>MSPISRHHHHHHLVPRGSASLRANDAPIVLLHGFTGWGREEMFGFKYWGGVRGDIEQWLNENGYRTYTLAVGPLSSNWDRACEAYAQLVGGTVDYGAAHAAKHGHARFGRTYPGLLPELKRGGRIHIIAHSQGGQNARMLVSLLENGSQEEREYAKAHNVSLSPLFEGGHHFVLSVTTIATPHDGTTLVNMVDFTDRFFDLQKAVLEAAAVASNVPYTSQVYDFKLDQWGLRRQPGESFDHYFDRLKRSPVWTSTDTARYDLSVSGALKLNQWVQASPNTYYLSFSTERTYRGALTGNHYPELGMNAFSAVVCAPFLGSYREPTLGIDDRWLENDGIVNTVSMNGPKRGSSDRIVPYDGTLKKGVWNDMGTYNVDHLEIIGVDPNPSFDIRAFYLRLAEQLASLRP[2x]

5M mutant lipase was derived through cumulative mutagenesis of amino acid residues (D43E/T118N/E226D/E250L/N304E) of T1 lipase from Geobacillus zalihae. Lipase (triacylglycerol acylhydrolase E.C.3.1.1.3) is a class of enzymes belonging to the serine hydrolases and is widely known as important biocatalysts. The active site of 5M is located at the center of the structure covered by two alpha-helices functioning as the lid.

The three-dimensional structure of 5M mutant lipase was solved at 2.64 Å with two molecules per asymmetric unit. The 5M crystal fitted the monoclinic system space group C2, signifying unit cell parameters of a = 117.59 Å, b = 81.27 Å, c = 99.52 Å. The 5M mutant lipase has a total of 21 α-helices and 11 β-sheets in its 3D crystal structures. The active sites of 5M mutant lipase composed of Ser113, His358, and Aps317. A similar composition of the catalytic triad was found in the crystal structure of Geobacillus thermoleovorans lipase. Both molecules in the asymmetric unit were highly similar, and the superimposition of alpha carbon atoms gave a root-mean-square deviation (RMSD) of 0.7789 Å. The zinc-binding sites in both chains composed of residues Asp61, Asp238, His87, and His81 in a tetrahedral formation. The calcium-binding site was coordinated by the residues Gly286, Glu360, Asp365, and Pro366. The mutations of amino acids in the 5M mutant caused the destruction of the ion interactions and hydrogen bonds inside the lipase structure, as shown by decreasing ion interactions and hydrogen bonds number. The mutant also experienced a decline in ion-pair interaction values, having only 20 pairs of ion interactions in chain A and 17 pairs of interactions in chain B. These results explained the loss in the thermostability of the 5M mutant, which also resulted in decreased melting temperature of this enzyme. The 5M lipase has a strong capability to catalyze long-chain carbon and shows preference towards pNP-C10.>[3x]MSLRYIVALTGGIGSGKSTVANAFADLGINVIDADIIARQVVEPGAPALHAIADHFGANMIAADGTLQRR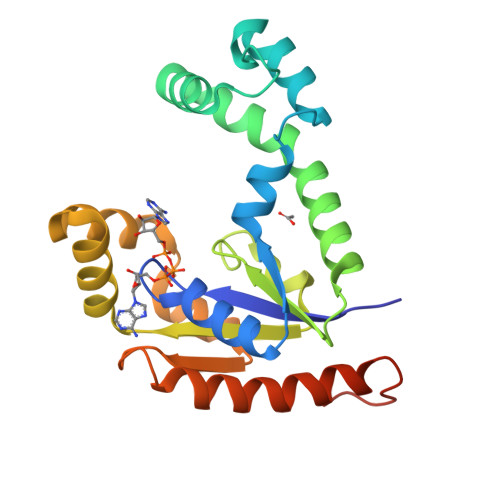ALRERIFANPEEKNWLNALLHPLIQQETQHQIQQATSPYVLWVVPLLVENSLYKKANRVLVVDVSPETQLKRTMQRDDVTREHVEQILAAQATREARLAVADDVIDNNGAPDAIASDVARLHAHYLQLASQFVSQEKPEGGSHHHHHH> EEMKKGHLERECMEETCSYEEAREVFEDSDKTNEFWNKYKDGDQCETSPCQNQGKCKDGLGEYTCTCLEGFEGKNCELFTKLCSLDNGDCDQFCHEEQNSVVCSCARGYTLADNG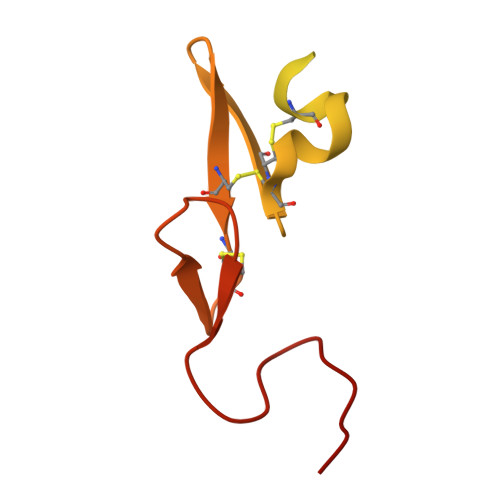KACIPTGPYPCGKQTLER2-(4-methylphenyl)-1,3-thiazole-4-carboxylic 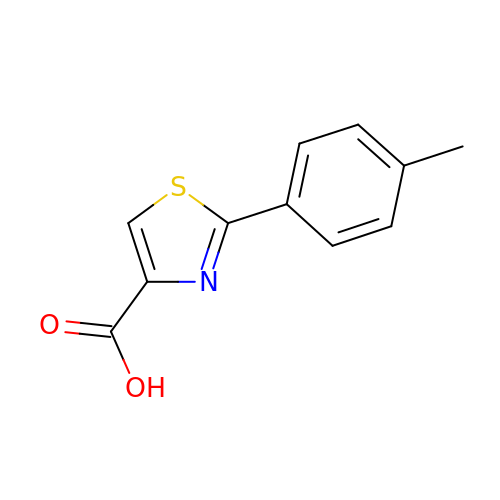acid | C11 H9 N O2 S | MTVWIZYQYPRZGZ-UHFFFAOYSA-N> CACGAGCCTGATCGGACAAGA;> AGGCAGCCTGTACGGACATCA;> AACCTACCTGGCAGGACGACTGCCTATGCTA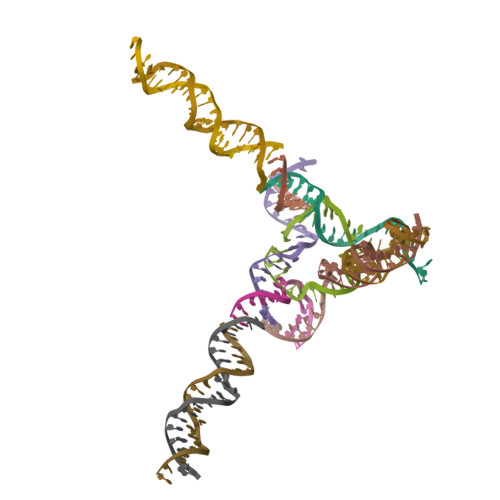;> GATCTTGTGGCTGC;> TTTAGCATAGGCAGTCGTGGCTCG;> ACTGATGTGGTAGG;> CACCGATCACCTGCCACCGTA;> CTTGCTGACGATCTAGCAGAG;> GTCTCTGCTAGATCGTCAGCA;> TGCTAGGCTAACTCGCTAGCG;> TCCGCTAGCGAGTTAGCCTAG trans-4-{2-[(1R)-1-hydroxyethyl]imidazo[4,5-d]pyrrolo[2,3-b]pyridin-1(6H)-yl}cyclohexanecarbonitrile | C17 H19 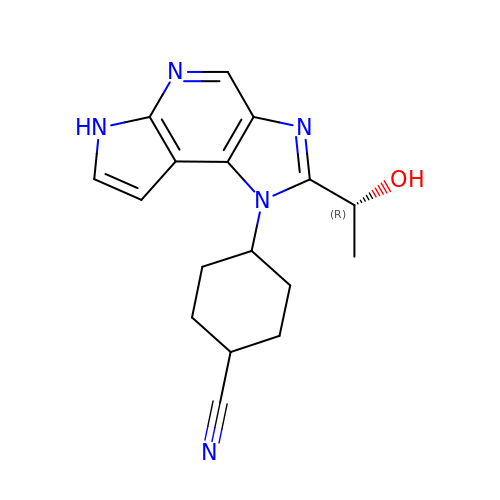N5 O | ANDWOIMHOOWCLK-IJLUTSLNSA-N GDE possesses the α-1,4 glucanotransferase (GT) and α-1,6 glucosidase (GC) activities, and removes glycogen phosphorylase-digested branches in two steps56. Its GT activity transfers a maltotriosyl group from the branch to a neighbouring non-reducing end, and forms an α-1,4 glycosidic bond between them. The last residue on the branch is subsequently removed by its GC activity. The structures revealed that CgGDE is composed of four domains, and adopts an elongated structure.

To study its interaction with glycogen, we also determined a complex structure of CgGDE with maltopentaose by the molecular replacement method. For the complex structure a GT-defective mutant (E564Q, see below) was used to protect maltopentaose from being converted to other oligosaccharides. In the maltopentaose complex crystal there are also two very similar protomers, both containing residues 3–1,528, and the r.m.s.d. for their related Cα atoms is 0.4 Å. The maltopentaose complex structure revealed a number of oligosaccharides bound at the GT and GC active sites, providing insights into their substrate recognition. At the GT active site two oligosaccharides, M and B (for mainchain and branch, respectively; see below), can be modelled into the electron densities, which contains 5 and 4 residues, respectively. Structural comparison with Taka-amylase A structure indicates that a glucose residue can fit into the space between residues B-1 and M5, suggesting the GT substrate mainchain and branch bind at where oligosaccharides M and B bind, respectively. At the GC domain active site an oligosaccharide with five residues can be fitted into the electron densities. It binds into a cleft, with residues 2–3 interacting with Asn1114, Leu1115, Arg1123, Asn1125 and Asp1207, residues 4–5 interacting with His1066, Trp1075, Tyr1407, Tyr1424 and Asp1503, and the C6 hydroxyl of its residue 4 pointing towards the active-site pocket. This suggests that the cleft and the active-site pocket accommodate the GC substrate mainchain and its single-residue branch, respectively. The maltopentaose complex structure revealed additional bound oligosaccharides. Our maltopentaose complex structure revealed highly specific substrate selectivity for the GT and GC active sites, which enables the GT active site to select glycogen phosphorylase-digested glycogen that contains four-residue branches, and the GC active site to select the GT reaction product that has a single-residue branch.

>[2x]MSAHRTLLLRLSDSGEPVTSCSYGQGVLTLPSLPLPQGKKLGDMPVYTVKLAIPAGSPVTRDGLIWTNCPPDFSTQFDREKFYKKIIKTSFHEDDHIDLDIYVPGTYCFYLSFKNDKDELETTRKFYFVVLPILSVNDKFIPLNSIAMQSVVSKWMGPTIKDWEKVFARVASKKYNMIHFTPLQHRGESNSPYSIYDQLEFDPTVFKSEKEVADMVERLRTEHNILSLTDIVFNHTANNSQWLLDHPEAGYNHKTSPHLISAIELDKKLLDFSEQMEALGYPVDLKTVDDLIKVMDGIKEHVIGELKLWEFYVVDVKQTVSELREKWGNSKSWSDDNIPSKDDSTNLAQFVRDNATEPGFGSLGERGSNKINIDKFAAILKKLHSEDYNNGIEELATKILNDINLPFYKEYDDDINEVLEQLFNRIKYLRIDDHGPKQGPITKKLPLSEPYFTRFKAKDGEEYALANNGWIWDGNPLVDFASSQSKAYLRREVIVWGDCVKLRYGKGPSDSPYLWERMSKYVEMNARIFNGFRIDNCHSTPLHVGQYFLDVARRVNPNLYVVAQLFSGSEAMDCLFVERLGISSLIREAMQAWSEEELSRLVHRHGGRPIGSYKFVPLDDFPYPADVKIDEEYCAYNPDDHSVKCVSEIMIPKTLTATPPHALFMDCTHDNETPNQKRTVEDTLPNAALVAFCSSAIGSVYGYDEVFPQLLDLVQEKRTYSCAENTGISKVKTLLNNMREEIASEAVDIEDSEMHVHHDGQYITFHRTNAKNGKGWYLVARTKFHSSGDQMLPRIKLSQTKATFKAAFSLERTGDAPISDEIIEGIPTKLRELTGFDIGFDENTKETSILLPQDFPQGSIVIFETQQLGIDDSLDHFIRSGAIKATEKLSLESINYVLYRAEQEEYDYSEGRSGAYDIPDYGKPVYCGLQGWVSILRKIIFYNDLAHPLSNNLRNGHWAVDYVVNRLDLYKDKEGVAEVQEWLRSRMERIKQLPSYLVPSFFALVVGIMYGCCRLRAMQLMSDNVGKSTVFVQSLAMTSIQMVSAMKSTSILPDQNIAAMAAGLPHFSTNYMRCWGRDVFISLRGLLLTTGRYEEAKEHILAFAKTLKHGLIPNLLDAGRNPRYNARDAAWFFVQAIQDYVTIVPGGVSLLQEKVTRRFPLDDEYIPYDDPKAFSYSSTIEEIIYEILNRHAGGIKYREANAGPNLDRVMKDEGFNVEVNVDWETGLIHGGSQFNCGTWMDKMGESEKANSVGVPGTPRDGAAVEINGLLKSCLRFVLQLSKDGKFKYTEVTKPDGSKISLSSWNDLLQENFERCFYVPKNKEDDNKFEIDATIINRRGIYKDLYRSGKPYEDYQFRPNFTIAMVVAPELFTPDYAAGAIELADQVLRGPVGMRTLDPSDYNYRPYYNNGEDSDDFATSKGRNYHQGPEWVWCYGYFIRAYHYFNFLTNPKCQVEGSAKKLKPSSYLYRKLYSRLLKHREWIENSPWAGLAELTNKDGEVCNDSSPTQAWSTGCLLDLFYDLWISYEE>[2x]MGSTAPLRLPVIDLSMKNLKPGTTSWNSVRTQVREALEEYGCFEAVIDAVSPELQKAVCNKGHELLNLPLETKMLNGNKPEYDGFTSIP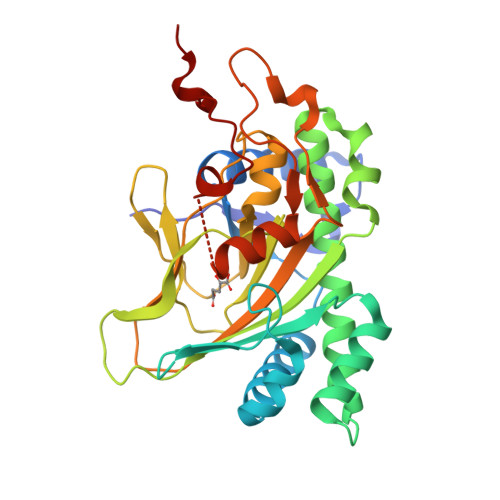NLNEGMGVGRITDLEKVERFTNLMWPEGNKDFCETVYSYGKRMAEVDHILKMMVFESFGMEKHFDSFCESTNYLLHFMRYQQPGKDGRSPALSLHKDKSILTIVNQNDVKGLEFETKDGEWILPTADNHIVLLGDCFMAWSNGRLHSPLHRVTLVANQARLSTSSFSFPKDIIETPAELVDEEHPLLFNPFEITELLAYCFTKEGAKAVCDLKQYKAYTGALEHHHHHH> HMKELKYDVLIIGGGFAGSSAA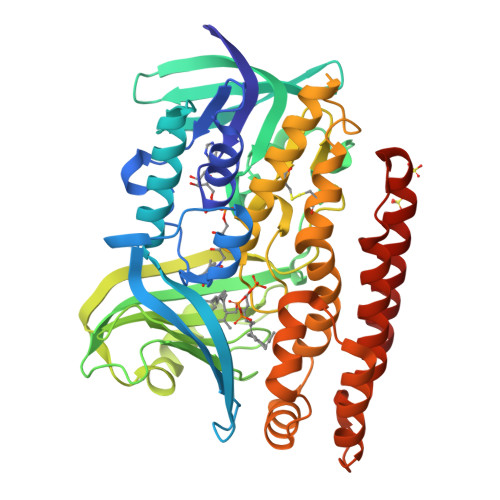YQLSRRGLKILLVDSKPWNRIGDKPCGDAVSKAHFDKLGMPYPKGEELENKINGIKLYSPDMQTVWTVNGEGFELNAPLYNQRVLKEAQDRGVEIWDLTTAMKPIFEDGYVKGAVLFNRRTNEELTVYSKVVVEATGYSRSFRSKLPPELPITEDLDDKDADVAYREVLLTKEDIEDHDYLRIFIDQETSPGGYWWYFPKGKNKVNVGLGIQGGMGYPSIHEYYKKYLDKYAPDVDKSKLLVKGGALVPTRRPLYTMAWNGIIVIGDSGFTVNPVHGGGKGSAMISGYCAAKAILSAFETGDFSASGLWDMNICYVNEYGAKQASLDIFRRFLQKLSNDDINYGMKKKIIKEEDLHEASEKGDLHLSVADKAMRVISGLGRPSLLFKLKAVAESMKKIKELYLNYPRSPSSLGSWRREVDNVLTEFNKSLS(4R)-4-hydroxy-4-(2-hydroxyphenyl)butanoic 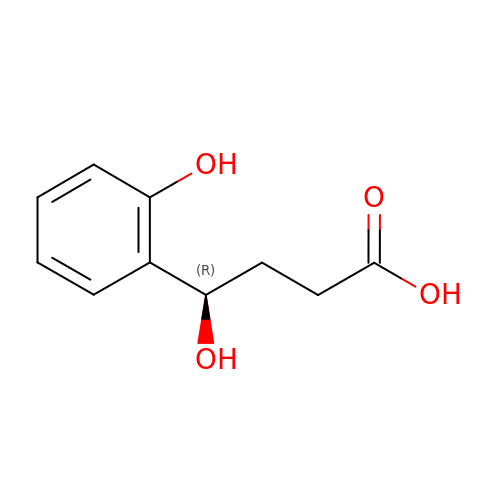acid | C10 H12 O4 | DHPGRNIALDCANN-SECBINFHSA-N[(1S,3R,4S)-3-amino-4-hydroxycyclopentyl]{(3R)-3-[(1S)-1-(biphenyl-2-yl)-1-hydroxy-5-methoxypentyl]piperidin-1-yl}methanone 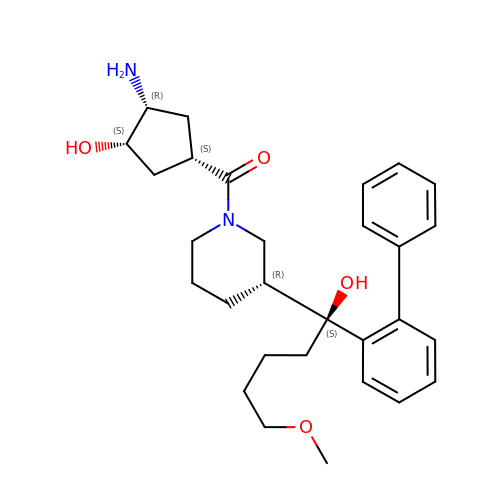| C29 H40 N2 O4 | GBAKDRIJFSDCNN-YJFNBJRFSA-N>MVRDMKHTVEVMIPEAEIKARIAELGRQITERYKDSGSDMVLVGLLRGSFMFMADLCREVQVSHEVDFMTASSYGSGMSTTRDLKILKDLDEDIRGKDVLIVEDIIDSGNTLSKVREILSLREPKSLAICTLLDKPSRREVNVPVEFIGFSIPDEFVVGYGIDYAQ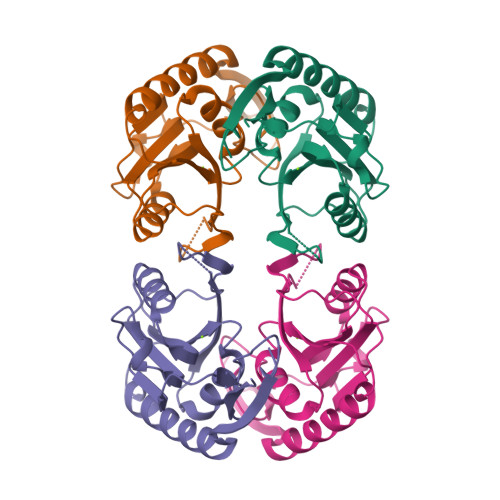RYRHLPYIGKVILLDE[2x]CYCLO-(GLYCINE-L-PROLINE) 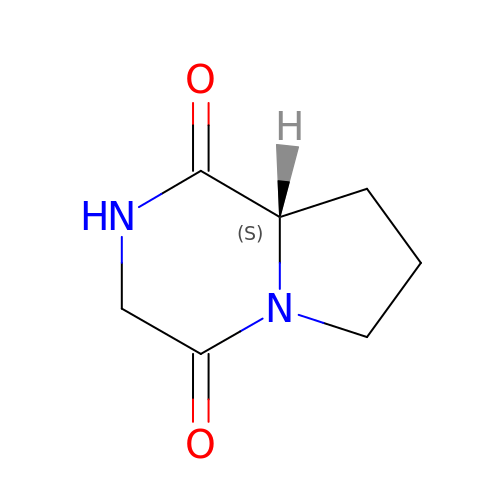INHIBITOR | C7 H10 N2 O2 | OWOHLURDBZHNGG-YFKPBYRVSA-N>[4x]MSNGILSQSIANMQQAEATIQSFSGLPQNAVNIQQNVGEVVAALLPQVQTMQQQVLAFAARLELQLTQQLANTGPFNPEALKAFVDLVQQEIAPIQTLTAQTLTA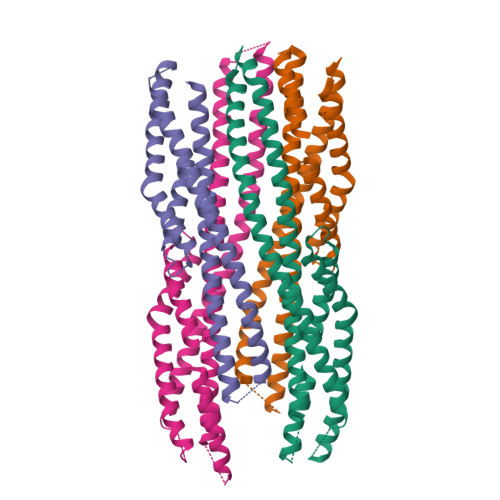SQSANDRITQDNIALQRIGVELQATIAGLQSNLDGARQELDSLNKKKLYLLGLGLLGLPGLIALAVTLTQTQNKVSSLEGQVNQIEGQIQRQQGFLGQTTAFSQQFGSLIDRVSKVGNTISLLGGDIANVARDAGQGDPELARLFFTAALTEVRTLQVDASLEHHHHHH>[6x]GGGHMILLKELKELFFLRTTYYLKKYNRSLPFGDMIVDRWDKAKLLGFGEGTSIYDSSIVLGEVKVGKDTWIGPNTILDGSGGGLIIGSNCSISAGVQIYTHDTVRKSLSGGKADID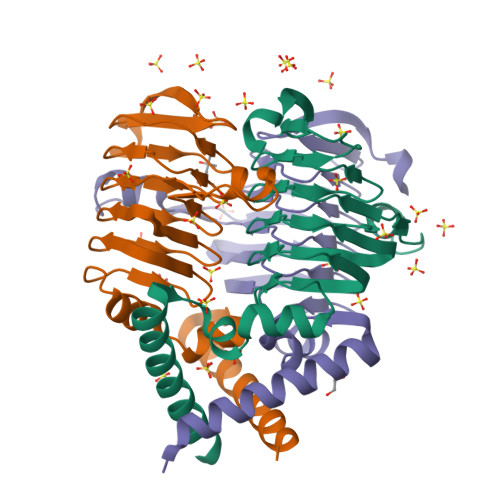KASTRIGSDCYLGPNTIIVKGVKIGDRVVVGANSLVLKDIPSDCKVFGSPAVIITDSLNYQRNNI> VLTEGNPRWEQTHLTYRIENYTPDLPRADVDHAIEKAFQLWSNVTPLTFTKVSEGQADIMISFVRGDHRDNSPFDGPGGNLAHAFQPGPGIGGDAHFDEDERWTNNFREYNLHRVAAHELGHSLGLSH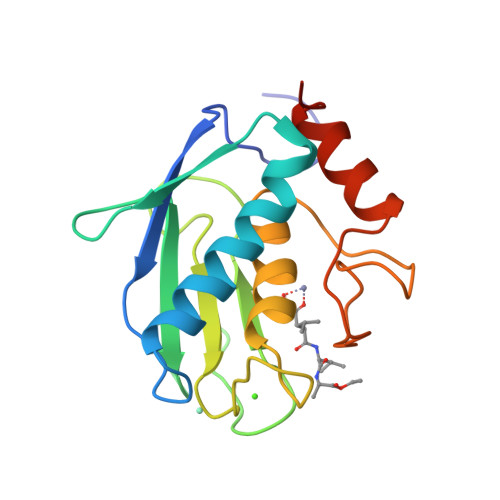STDIGALMYPSYTFSGDVQLAQDDIDGIQAIYGRSQNPVQP> MSRQASRLDAKKVNSEFLTLTYGALVTQMLRDFENAEDVNKQLERIGY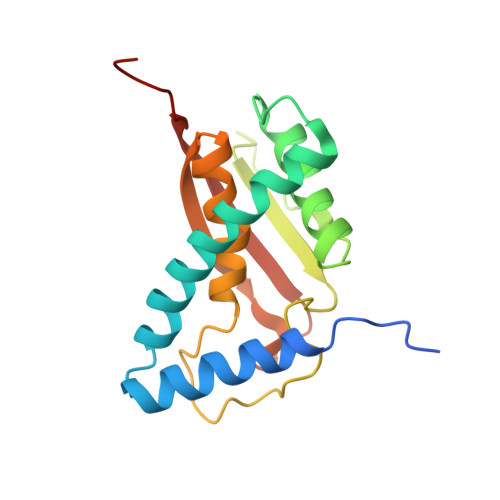NMGMRLIEDFLARTSAPRCLEMRETADRIQQAFRIYLNIQPTISNWSPASDEFSLVFDSNPLTEFVELPPDLTNLRYSAILSGCIRGALEMVQLEVQCWFVQDQLKGDNVTELRVKFVRRLEEVIPAGED>[2x]RAPAPATPHAPDHSPAPNSPTLTRPPEGPKFPRVKNWELGSITYDTLCAQSQQDGPCTPRRCLGSLVLPRKLQTRPSPGPPPAEQLLSQARDFINQYYSSIKRSGSQAHEERLQEVEAEVASTGTYHLRESELVFGAKQAWRNAPRCVGRIQWGKLQVFDARDCSSAQEMFTYICNHIKYATNRGNLRSAITVFPQRAPGRGDFRIWNSQLVRYAGYRQQDGSVRGDPANVEITELCIQHG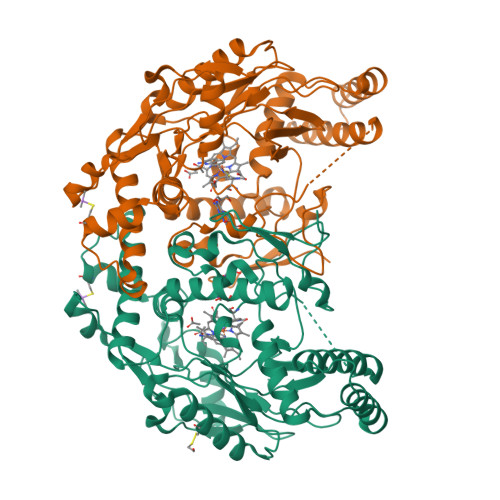WTPGNGRFDVLPLLLQAPDEAPELFVLPPELVLEVPLEHPTLEWFAALGLRWYALPAVSNMLLEIGGLEFSAAPFSGWYMSTEIGTRNLCDPHRYNILEDVAVCMDLDTRTTSSLWKDKAAVEINLAVLHSFQLAKVTIVDHHAATVSFMKHLDNEQKARGGCPADWAWIVPPISGSLTPVFHQEMVNYILSPAFRYQPDPW> MSSAIKEVQGAPVKWVTNWTPEAIRGLVDQEKGLLDPRIYADQSLYELELERVFGRSWLLLGHESHVPETGDFLATYMGEDPVVMVRQKDKSIKVFLNQCRHRGMRICRSDAGNAKAFTCSYHGWAYDIAGKLVNVPFEKEAFCDKKEGDCGFDKAEWGPLQARVATYKGLVFANWDVQAPDLETYLGDARPYMDVMLDRTPAGTVAIGGMQKWVIPCNWKFAAEQFCSDMYHAGTTTHLSGILAGIPPEMDLSQAQIPTKGNQFRAAWGGHGSGWYVDEPGSLLAVMG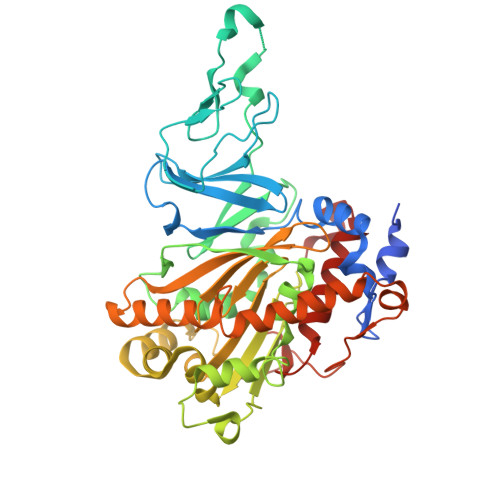PKVTQYWTEGPAAELAEQRLGHTGMPVRRMVGQHMTIFPTCSFLPGINTIRTWHPRGPNEIEVWAFTLVDADAPAEIKEEYRRHNIRNFSAGGVFEQDDGENWVEIQKGLRGYKAKSQPLNAQMGLGRSQTGHPDFPGNVGYVYAEEAARGMYHHWMRMMSEPSWATLKP> MAHHHHHHMKEVFIVSAVRTPMGSFMGSLSGVPATQLGAVAIKGALDKINLNPAEIQDVYMGNVLQAGEGQAPAKQAALGAGLPNTTPTTAVNKVCASGMKAVMMAAQAVKAGDVEAIVAGGMENMSQVPHYIDGRNGVKLGDIKLQDGLLKDGLTDVYSKQHMGNCAELCAKEYNITREEQDAFA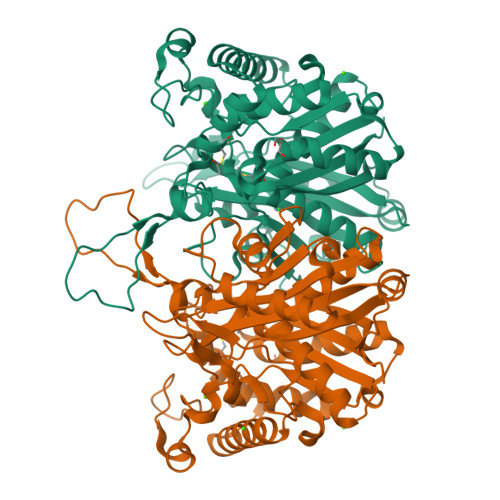IQSYERSAKAWSEGKFKEEVVPVSIPQRKGEPIIFAEDEEYKNVKFDRIPTLPTVFQKENGTVTAANASTLNDGASALVLMSKEKMESLGLKPLAKIVSYADAAQAPEWFTTAPAKALPIALAKANLTINDIDFFEFNEAFSVVGLANNKILGLDAAKVNVNGGAVALGHPLGSSGSRIIVTLINVLKQNNAKYGAAAICNGGGGASAIVIENIK> MKIFSVRQTVLPALLVLSPVVFAADEQTMIVSAAPQVVSELDTPAAVSVVDGEEMRLATPRINLSESLTGVPGLQVQNRQNYAQDLQLSIRGFGSRSTYGIRGIRLYVDGIPATMPDGQGQTSNIDLSSVQNVEVLRGPFSALYGNASGGVMNVTTQTGQQPPTIEASSYYGSFGSWRYGLKATGATGDGTQPGDVDYTVSTTRFTTHGYRDHSGAQKNLANAKLGVRIDEASKLSLIFNSVDIKADDPGGLTKAEWKANPQQAPRAEQYDTRKTIKQTQAGLRYERSLSSRDDMSVMMYAGERETTQYQSIPMAPQLNPSHAGGVITLQRHYQGIDSRWTHRGELGVPVTFTTGLNYENMSENRKGYNNFRLNSGMPEYGQKGELRRDERNLMWNIDPYLQTQWQLSEKLSLDAGVRYSSVWFDSNDHYVTPGNGDDSGDASYHKWLPAGSLKYAMTDAWNIYLAAGRGFETPTINELSYRADGQSGMNLGLKPSTNDTIEIGSKTRIGDGLLSLALFQTDTDDEIVVDSSS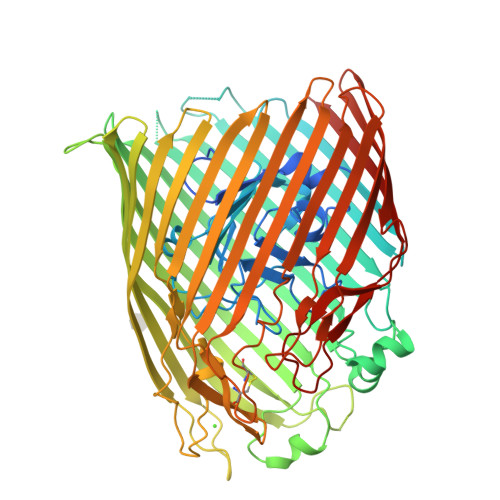GGRTTYKNAGKTRRQGAELAWDQRFAGDFRVNASWTWLDATYRSNVCNEQDCNGNRMPGIARNMGFASIGYVPEDGWYAGTEARYMGDIMADDENTAKAPSYTLVGLFTGYKYNYHNLTVDLFGRVDNLFDKEYVGSVIVNESNGRYYEPSPGRNYGVGMNIAWRFE> QAQITGRPEWIWLALGTALMGLGTLYFLVKGMGVSDPDAKKFYAITTLVPAIAFTMYLSMLLGYGLTMVPFGGEQNPIYWARYADWLFTTPLLLLDLALLVDADQGTILAAVGADGIMIGTGLVGALTKVYSYRFVWWAISTAAMLYILYVLFFGFTSKAESMRPEVASTFKVLRNVTVVLWSAYPVVWLIGSEGAGIVPLNIETLLFMVLDVSAKVGFGLILLRSR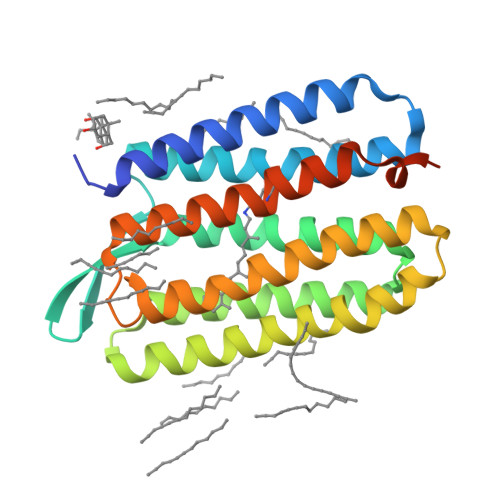AIFGEAEAPEPSAGDGAAATSD> MDAPEEEDHVLVLRKSNFAEALAAHKYLLVEFYAPWCGHCKALAPEYAKAAGKLKAEGSEIRLAKVDATEESDLAQQYGVRGYPTIKFFRNGDTASPKEYTAGREADDIVNWLKKRTGPAATTLPDG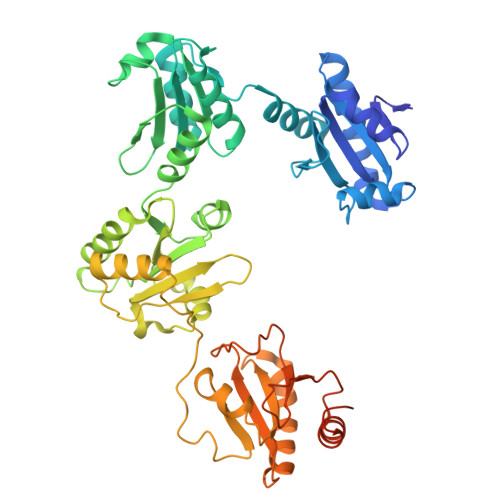AAAESLVESSEVAVIGFFKDVESDSAKQFLQAAEAIDDIPFGITSNSDVFSKYQLDKDGVVLFKKFDEGRNNFEGEVTKENLLDFIKHNQLPLVIEFTEQTAPKIFGGEIKTHILLFLPKSVSDYDGKLSNFKTAAESFKGKILFIFIDSDHTDNQRILEFFGLKKEECPAVRLITLEEEMTKYKPESEELTAERITEFCHRFLEGKIKPHLMSQELPEDWDKQPVKVLVGKNFEDVAFDEKKNVFVEFYAPWCGHCKQLAPIWDKLGETYKDHENIVIAKMDSTANEVEAVKVHSFPTLKFFPASADRTVIDYNGERTLDGFKKFLESGGQDGAGDDDDLEDLEEAEEPDMEEDDDQKAVKDEL> HLSDMLQQLHSVNASKPSERGLVRQEEAEDPACIPIFWVSKWVDYSDKYGLGYQLCDNSVGVLFNDS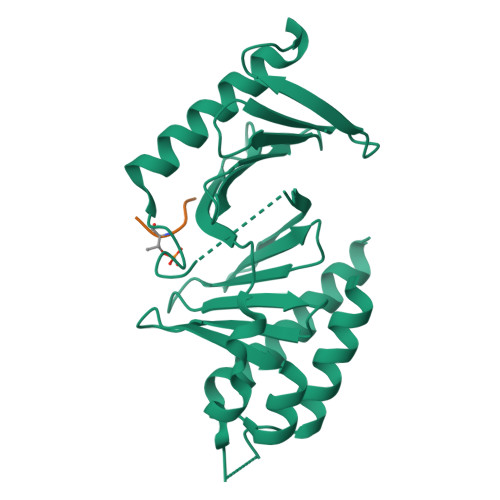TRLILYNDGDSLQYIERDGTESYLTVSSHPNSLMKKITLLKYFRNYMSEHLLKAGANITPREGDELARLPYLRTWFRTRSAIILHLSNGSVQINFFQDHTKLILCPLMAAVTYIDEKRDFRTYRLSLLEEYGCCKELASRLRYARTMVDKLLSSR;> VLSTLX>MKHSLPDLPYDYGALEPHINAQIMQLHHSKHHAAYVNNLNVTEEKYQEALAKGDVTAQIALQPALKFNGGGHINHSIFWTNLSPNGGGEPKGELLEAIKRDFGSFDKFKEKLTAASVGVQGSGWGWLGFNKERGHLQIAACPNQDPLQGTTGLIPLLGIDVFEHAYYLQYKNVRPDYLKAIWNVINWENVTERYMACKK[2x]

Human manganese superoxide dismutase (MnSOD) is a crucial oxidoreductase that maintains the vitality of mitochondria by converting superoxide (O2●−) to molecular oxygen (O2) and hydrogen peroxide (H2O2) with proton-coupled electron transfers (PCETs). Human MnSOD has evolved to be highly product inhibited to limit the formation of H2O2, a freely diffusible oxidant and signaling molecule. The Mn ion is bound by inner-sphere residues His26, His74, His163, Asp159, and a solvent molecule denoted as WAT1. The hydrogen bond network extends from WAT1 to outer-sphere residues Gln143, Tyr34, another solvent molecule denoted as WAT2, His30, and Tyr166 from the neighboring subunit.

For these reasons, we used H2O2 soaking in combination with the Trp161Phe MnSOD variant to characterize the inhibited complex. To visualize the atomic identity of the product-inhibited complex and the corresponding active site protonation states, a cryocooled neutron structure of perdeuterated Trp161Phe MnSOD soaked with deuterium peroxide (D2O2) was solved at 2.30 Å resolution. For chain B of the D2O2-soaked neutron structure, two dioxygen species are found within the active site. One of the dioxygen species is singly-protonated and bound directly to the metal ion, replacing the position of WAT1, and forming a SSHB with Gln143 that is in the neutral form. In the same active site, D2O2 is observed binding tightly between an ionic Tyr34 and neutral His30. While the D2O2 binding site between His30 and Tyr34 was predicted, the neutron structure is the first experimental evidence for this binding. For chain A of the D2O2-soaked neutron structure, the active site is reduced, but a dioxygen ligand is not present, and Gln143 is deprotonated. Our radiation-free neutron diffraction suggests that product inhibition in human MnSOD is a five-coordinate complex with a singly-protonated dioxygen ligand displacing the metal-bound solvent molecule. Although sterically crowded, this complex prohibits catalysis during its lifetime by blocking the fast back-and-forth proton transfer between WAT1 and Gln143 during PCET redox cycling. Our XAS measurements and DFT simulations support the interpretation that the Mn ion is divalent and the singly-protonated dioxygen species is HO2−.> EPLAAGAVILRRFAFNAAEQLIRDINDVASQSPFRQMVTPGGYTMSVAMTNCGHLGWTTHRQGYLYSPIDPQTNKPWPAM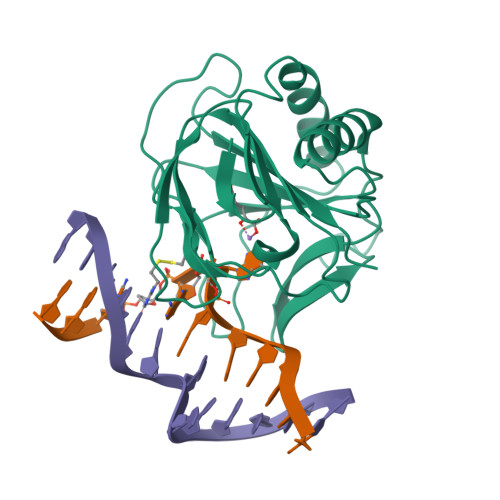PQSFHNLCQRAATAAGYPDFQPDACLINRYAPGAKLCLHQDKDEPDLRAPIVSVSLGLPAIFQFGGLKRNDPLKRLLLEHGDVVVWGGESRLFYHGIQPLKAGFHPLTIDCRYNLTFRQAG> MAPQIRSRSLAAQEPASVLEEARLRLHVSAVPESLPCREQEFQDIYNFVESKLLDHTGGCMYISGVPGTGKTATVHEVIRCLQQAAQANDVPPFQYIEVNGMKLTEPHQVYVQILQKLTGQKATANHAAELLAKQFCTRGSPQETTVLLVDELDLLWTHKQDIMYNLFDWPTHKEARLVVLAIANTMDLPERIMMNRVSSRLGLTRMCFQPYTYSQLQQILRSRLKHLKAFEDDAIQLVARKVAALSGDARRCLDICRRATEICEFSQQKPDSPGLVTIAHSMEAVDEMFSSSYITAIKNSSVLEQSFLRAILAEFRRSGLEEATFQQIYSQHVALCRMEGLPYPTMSETMAVCSHLGSCRLLLVEPSRNDLLLRVRLNVSQDDVLYALKDE;> MSKPELKEDKMLEVHFVGDDDVLNHILDREGGAKLKKERAQLLVNPKKIIKKPEYDLEEDDQEVLKDQNYVEIMGRDVQESLKNGSATGGGNKVYSFQNRKHSEKMAKLASELAKTPQKSVSFSLKNDPEITINVPQSSKGHSASDKVQPKNNDKSEFLSTAPRSLRKRLIVPRSHSDSESEYSASNSEDDEGVAQEHEEDTNAVIFSQKIQAQNRVVSAPVGKETPSKRMKRDKTSDLVEEYFEAHSSSKVLTSDRTLQKLKRAKLDQQTLRNLLSKVSPSFSAELKQLNQQYEKLFHKWMLQLHLGFNIVLYGLGSKRDLLERFRTTMLQDSIHVVINGFFPGISVKSVLNSITEEVLDHMGTFRSILDQLDWIVNKFKEDSSLELFLLIHNLDSQMLRGEKSQQIIGQLSSLHNIYLIASIDHLNAPLMWDHAKQSLFNWLWYETTTYSPYTEETSYENSLLVKQSGSLPLSSLTHVLRSLTPNARGIFRLLIKYQLDNQDNPSYIGLSFQDFYQQCREAFLVNSDLTLRAQLTEFRDHKLIRTKKGTDGVEYLLIPVDNGTLTDFLEKEEEEA;> MATSSMSKGCFVFKPNSKKRKISLPIEDYFNKGKNEPEDSKLRFETYQLIWQQMKSENERLQEELNKNLFDNLIEFLQKSHSGFQKNSRDLGGQIKLREIPTAALVLGVNVTDHDLTFGSLTEALQNNVTPYVVSLQAKDCPDMKHFLQKLISQLMDCCVDIKSKEEESVHVTQRKTHYSMDSLSSWYMTVTQKTDPKMLSKKRTTSSQWQSPPVVVILKDMESFATKVLQDFIIISSQHLHEFPLILIFGIATSPIIIHRLLPHAVSSLLCIELFQSLSCKEHLTTVLDKLLLTTQFPFKINEKVLQVLTNIFLYHDFSVQNFIKGLQLSLLEHFYSQPLSVLCCNLPEAKRRINFLSNNQCENIRRLPSFRRYVEKQASEKQVALLTNERYLKEETQLLLENLHVYHMNYFLVLRCLHKFTSSLPKYPLGRQIRELYCTCLEKNIWDSEEYASVLQLLRMLAKDELMTILEKCFKVFKSYCENHLGSTAKRIEEFLAQFQSLDAETKEEEDASGSQPKGLQKTDLYHLQKSLLEMKELRRSKKQTKFEVLRENVVNFIDCLVREYLLPPETQPLHEVVYFSAAHALREHLNAAPRIALHTALNNPYYYLKNEALKSEEGCIPNIAPDICIAYKLHLECSRLINLVDWSEAFATVVTAAEKMDANSATSEEMNEIIHARFIRAVSELELLGFIKPTKQKTDHVARLTWGGC;> MSSRKSKSNSLIHTECLSQVQRILRERFCRQSPHSNLFGVQVQYKHLSELLKRTALHGESNSVLIIGPRGSGKTMLINHALKELMEIEEVSENVLQVHLNGLLQINDKIALKEITRQLNLENVVGDKVFGSFAENLSFLLEALKKGDRTSSCPVIFILDEFDLFAHHKNQTLLYNLFDISQSAQTPIAVIGLTCRLDILELLEKRVKSRFSHRQIHLMNSFGFPQYVKIFKEQLSLPAEFPDKVFAEKWNENVQYLSEDRSVQEVLQKHFNISKNLRSLHMLLMLALNRVTASHPFMTAVDLMEASQLCSMDSKANIVHGLSVLEICLIIAMKHLNDIYEEEPFNFQMVYNEFQKFVQRKAHSVYNFEKPVVMKAFEHLQQLELIKPMERTSGNSQREYQLMKLLLDNTQIMNALQKYPNCPTDVRQWATSSLSWL;> MPHLENVVLCRESQVSILQSLFGERHHFSFPSIFIYGHTASGKTYVTQTLLKTLELPHVFVNCVECFTLRLLLEQILNKLNHLSSSEDGCSTEITCETFNDFVRLFKQVTTAENLKDQTVYIVLDKAEYLRDMEANLLPGFLRLQELADRNVTVLFLSEIVWEKFRPNTGCFEPFVLYFPDYSIGNLQKILSHDHPPEYSADFYAAYINILLGVFYTVCRDLKELR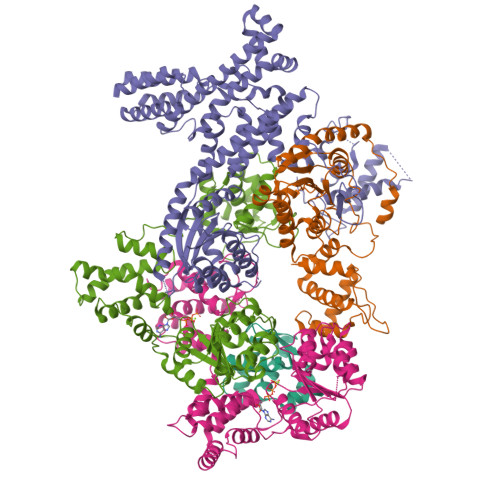HLAVLNFPKYCEPVVKGEASERDTRKLWRNIEPHLKKAMQTVYLREISSSQWEKLQKDDTDPGQLKGLSAHTHVELPYYSKFILIAAYLASYNPARTDKRFFLKHHGKIKKTNFLKKHEKTSNHLLGPKPFPLDRLLAILYSIVDSRVAPTANIFSQITSLVTLQLLTLVGHDDQLDGPKYKCTVSLDFIRAIARTVNFDIIKYLYDFL2-morpholin-4-ylaniline 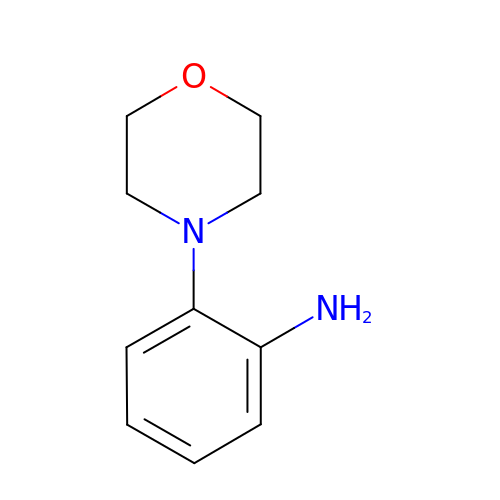| C10 H14 N2 O | QKWLVAYDAHQMLG-UHFFFAOYSA-N> RSPWQGTLPPFLPCELQPHGLVNCNWLFLKSVPHFSAAAPRDNVTSLSLLSNRIHHLHDSDFAQLSNLQKLNLKWNCPPAGLSPMHFPCHMTIEPNTFLAVPTLEELNLSYNGITTVPALPSSLVSLILSRTNILQLDPTSLTGLHALRFLYMDGNCYYKNPCGRALEVAPGALLGLGNLTHLSLKYNNLTTVPRSLPPSLEYLLLSYNHIVTLAPEDLANLTALRVLDVGGNCRRCDHARNPCVECPHKFPQLHSDTFSHLSRLEGLVLKDSSLYQLNPRWFRGLGNLTVLDLSENFLYDCITKTKAFQGLAQLRRLNLSFNYHKKVSFAHLTLAPSFGSLLSLQELDMHGIFFRSLSQKTLQPLARLPMLQRLYLQMNFINQAQLGIFKDFPGLRYIDLSDNRISGAVEPVATTGEVDGGKKVWLTSRDLTPGPLDTPSSEDFMPSCKNLSFTLDLSRNNLVTVQPEMFAQLSRLQCLRLSHNSISQAVNGSQFVPLTSLQVLDLSHNKLDLYHGRSFTELPRLEALDLSYNSQPFSMRGVGHNLSFVAQLPTLRYLSLAHNGIHSRVSQQLCSTSLWALDFSGNSLSQMWAEGDLYLRFFQGLRSLIRLDLSQNRLHTLLPCTLGNLPKSLQLLRLRNNYLAFF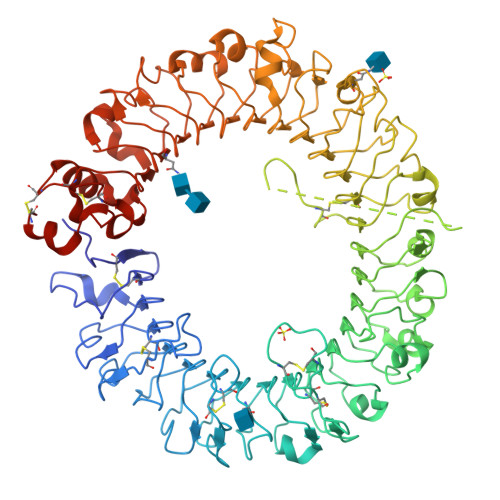NWSSLTLLPNLETLDLAGNQLKALSNGSLPSGTQLQRLDVSRNSIIFVVPGFFALATRLRELNLSANALRTVEPSWFGFLAGSLEVLDVSANPLHCACGAAFVDFLLQVQAAVPGLPSRVKCGSPGQLQGRSIFAQDLRLCLDESLSWDEFLVPR2ALPHA-(3-HYDROXYPROPOXY)-1ALPHA,25-DIHYDROXYVITAMIN D3 | C30 H50 O5 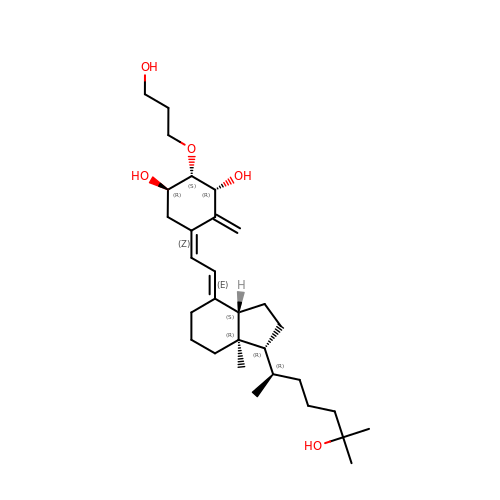| FZEXGDDBXLBRTD-VCBASKJSSA-N>MGSHHHHHHENLYFQGHMNSFYSQEELKKIGFLSVGKNVLISKKASIYNPGVISIGNNVRIDDFCILSGKVTIGSYSHIAAYTALYGGEVGIEMYDFANISSRTIVYAAIDDFSGNALMGPTIPNQYKNVKTGKVI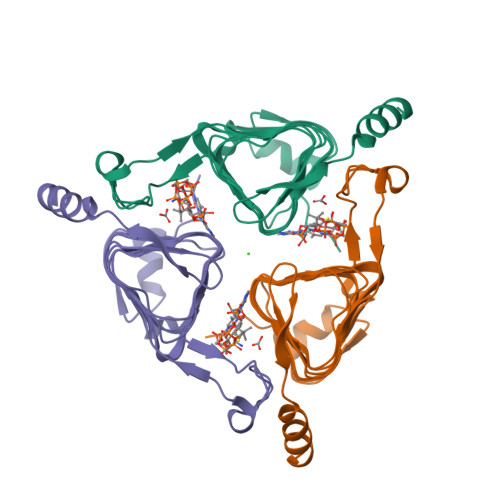LKKHVIIGAHSIIFPNVVIGEGVAVGAMSMVKESLDDWYIYVGVPVRKIKARKRKIVELENEFLKSMNS[3x]>[4x]MAHHHHHHMDQIKIEENATGFSYESLFREYLNETVTEVWIEDPYIRHTHQLYNF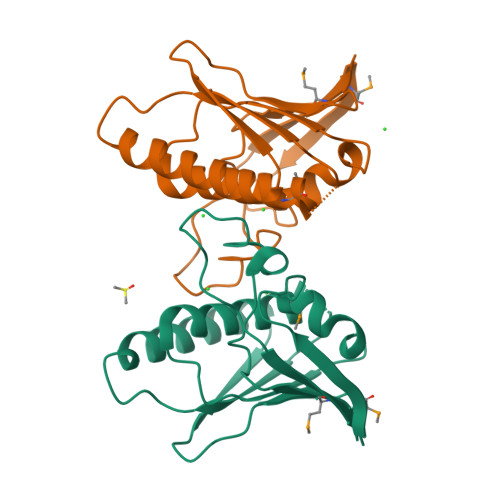LRFCEMLIKRPCKVKTIHLLTSLDEGIEQVQQSRGLQEIEESLRSHGVLLEVQYSSSIHDREIRFNNGWMIKIGRGLDYFKKPQSRFSLGYCDFDLRPCHETTVDIFHD>MKTPEDCTGLADIREAIDRIDLDIVQALGR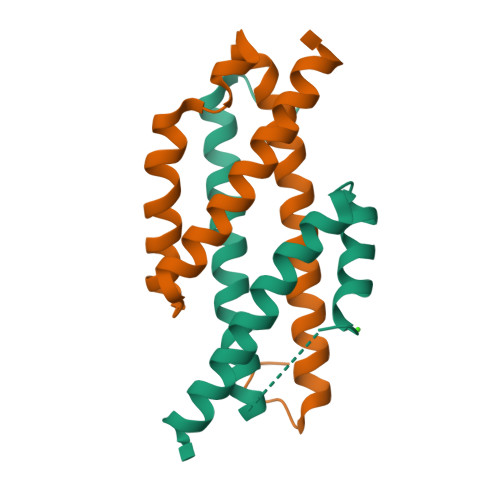RMDYVKAASRFKASEAAIPAPERVAAMLPERARWAEENGLDAPFVEGLFAQIIHWYTAEQIKYWRQTRGAA[4x]> QSACTLQSETHPPLTWQKCSSGGTCTQQTGSVVIDANWRWTHATNSSTNCYDGNTWSSTLCPDNETCAKNCCLDGAAYASTYGVTTSGNSLSIDFVTQSAQKNVGARLYLMASDTTYQEFTLLGNEFSFDVDVSQLPCGLNGALYFVSMDADGGVSKYPTNTAGAKYGTGYCDSQCPRDLKFINGQANVEGWEPSSNNANTGIGGHGSCCSEMDIWEANSISEALTPHPCTTVGQEI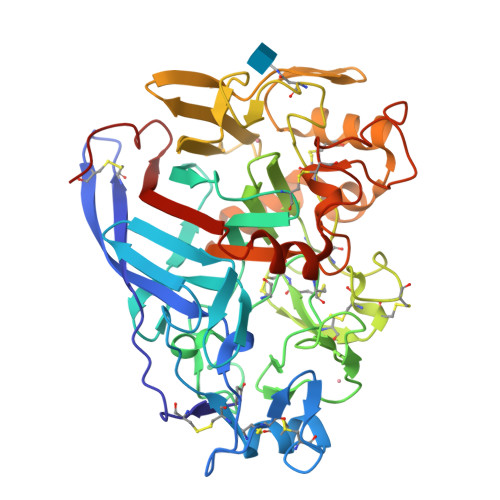CEGCGCGGTYSCNRYGGTCDPDGCDWNPYRLGNTSFYGPGSSFTLDTTKKLTVVTQFETSGAINRYYVQNGVTFQQPNAELGSYSGNELNDDYCTAEEAEFGGSSFSDKGGLTQFKKATSGGMVLVMSLWDDYYANMLWLDSTYPTNETSSTPGAVRGSCSTSSGVPAQVESQSPNAKVTFSNIKFGPIGSTGNPSG>SNAMQKINIDRHATAQINMLANKLMLKSSTAYTQKFGIGMTEWRIISVLSSASDCSVQKISDILGLDKAAVSRTVKKLEEKKYIEVNGHSEDKRTYAIN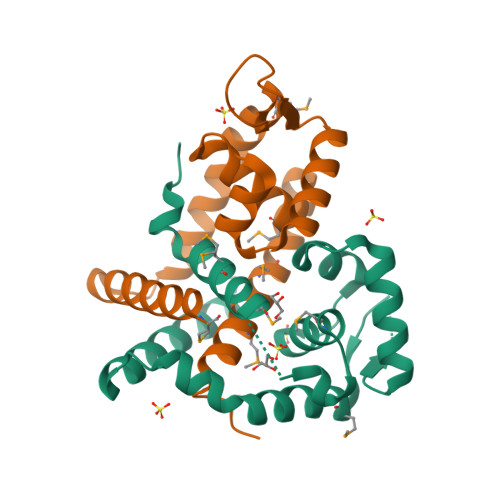LTEMGQELYEVASDFAIEREKQLLEEFEEAEKDQLFILLKKLRNKVDQM[4x]2-{[4-amino-3-(3-fluoro-4-hydroxyphenyl)-1H-pyrazolo[3,4-d]pyrimidin-1-yl]methyl}-5-methyl-3-(2-methylphenyl)quinazolin-4(3H)-one 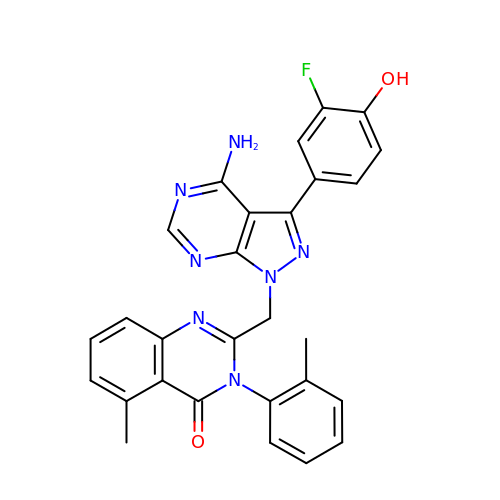| C28 H22 F N7 O2 | TYLTZPAGUBOPCU-UHFFFAOYSA-N> GSHMKNSVSVDLPGSMKVLVSKSSNADGKYDLIATVDALELSGTSDKNNGSGVLEGVKADASKVKLTISDDLGQTTLEVFKSDGSTLVSKKVTSKDKSSTYELFNEKGELSAKYITRADKSSTYELFNEKGELSAKYITRADKSSTYELFNEKGELSFKYITRADKSSTYELFNEKGELSFKYITRADGTRLEYTGIKSDGSGKAKEVLKGYVLEGTLTAEKTTLVVKEGTVTLSKNISKSGEVSVELNDTDSSAATKKTAAWNSGTSTLTITVNSKKTKDLVFTSSNTITVQQYDSNGTSLEGSAV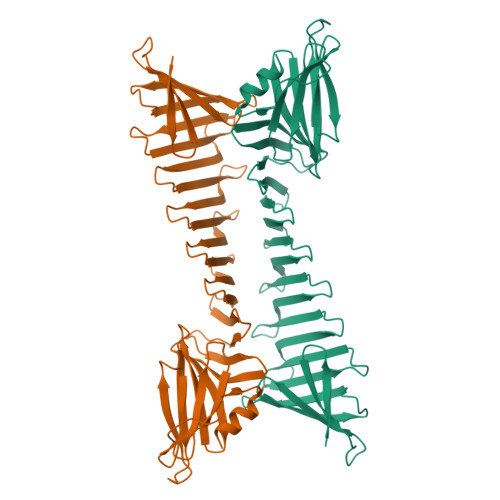EITKLDEIKNALK>[3x]XMEMLTKFESRSSRAKGVAFHPTQPWILTSLHNGRIQLWDYRMGTLLDRFDGHDGPVRGIAFHPTQPLFVSGGDDYKVNVWNYKSRKLLFSLCGHMDYVRVCTFHHEYPWILSCSDDQTIRIWNWQSRNCIAILTGHSHYVMCAAFHPSEDLIVSASLDQTVRVWDISGLRMKNAAPVSMSK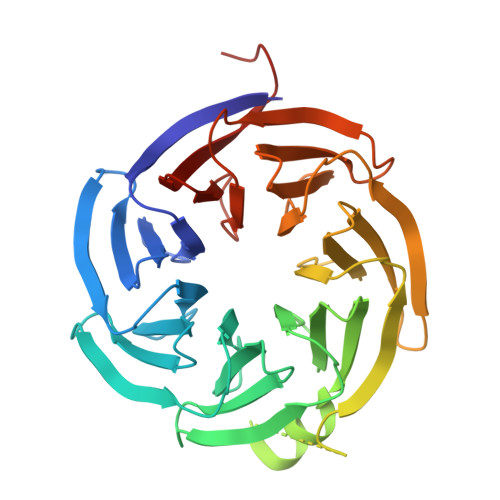EDQKAQAHNSKSNDKKGSTDAIVKFVLEGHDRGVNWCAFHPTLPLILSAGDDRLVKLWRMTASKAWEVDTCRGHFNNVSCCLFHPHQELILSASEDKTIRVWDLNRRTAVQTFRRDNDRFWFITVHPKLNLFAAAHDSGVMVFKLESAWSHPQFEK> MDLTNKNVIFVAALGGIGLDTSRELVKRNLKNFVILDRVENPTALAELKAINPKVNITFHTYDVTVPVAESKKLLKKIFDQLKTVDILINGAGILDDHQIERTIAINFTGLVNTTTAILDFWDKRKGGPGGIIANICSVTGFNAIHQVPVYSASKAAVVSFTNSLAKLAPITGVTAYSINPGITRTPLV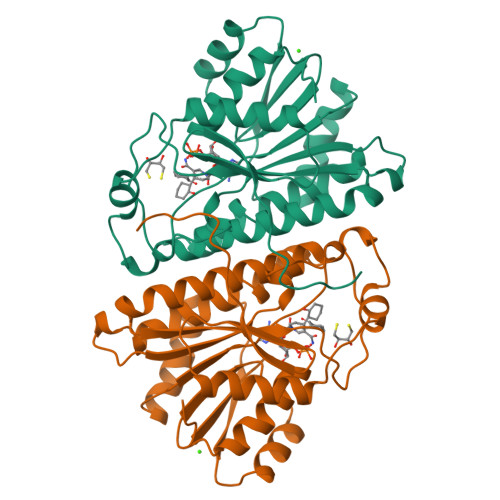HTFNSWLDVEPRVAELLLSHPTQTSEQCGQNFVKAIEANKNGAIWKLDLGTLEAIEWTKHWDSHI5-[(6R)-5-ethanoyl-4-methyl-2-oxidanylidene-3-[3-(trifluoromethyl)phenyl]-1,6-dihydropyrimidin-6-yl]pyridine-2-carbonitrile | C20 H15 F3 N4 O2 | 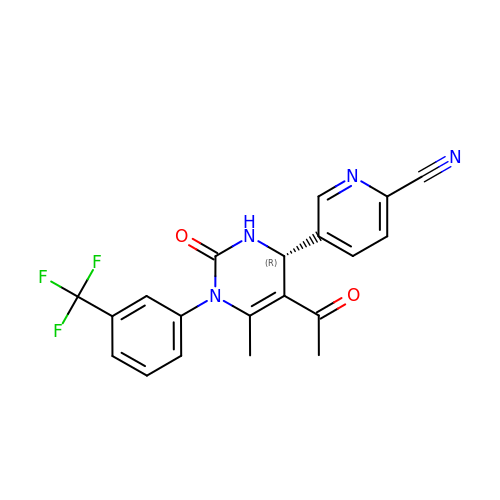PGIVGIFOWOVINL-GOSISDBHSA-N> TFRMRIYERDDFRGQMSEITDDCPSLQDRFHLTEVHSLNVLEGSWVLYEMPSYRGRQY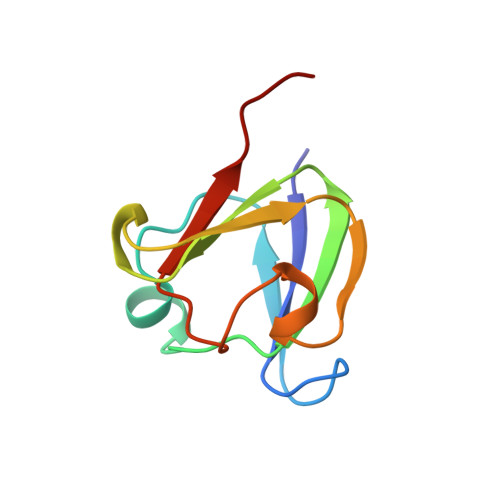LLRPGEYRRYLDWGAMNAKVGSLRRVMDFY3-O-methyl-beta-D-glucopyranose | C7 H14 O6 | 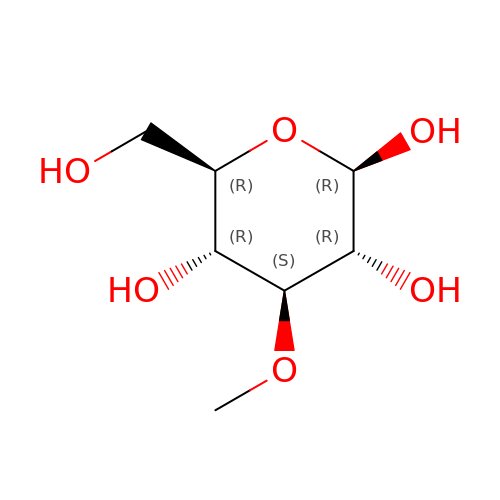SCBBSJMAPKXHAH-BNWJMWRWSA-N>ELGSLIRATNLWGYTDLMRELGADPLPFLRRFDIPPGIEHQEDAFMSLAGFVRMLEASAAELDCPDFGLRLARWQGLGILGPVAVIARNAATLFGGLEAIGRYLYVHSPALTLTVSSTTARSNVRFGYEVTEPGIPYPLQGYELSMANAARMIRLLGGPQARARVFSFRHAQLGTDAAYREALGCT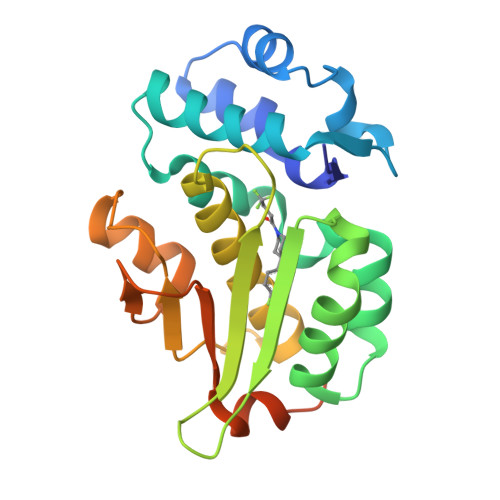VRFGRTWCGFEVDHRLAGRPIDHADPETKRIATKYLESQYLPS[2x]> GSHMASMKKKGSVVIVGRINLSGDTAYAQQTRGEEGCQETSQTGRDKNQVEGEVQIVSTATQTFLATSINGVLWTVYHGAGTRTIASPKGPVTQMYTNVDKDLVGWQAPQGSRSLTPCTCGSSDLYLVTRHADVIPVRRRGDSRGSLLSPRPISYLKGSSGGPLLCPAGHAVGIFRTAV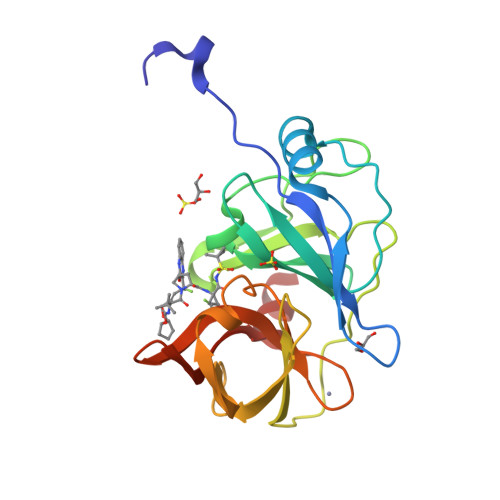CTRGVAKAVDFIPVESLETTMRSP>MHHHHHHMGDALGLIETKGLVACIEAADAMCDAANVELIGYENVGSGLVTAMVKGDVGAVKAAVDSGVESAQRIGEVVTSLVIARP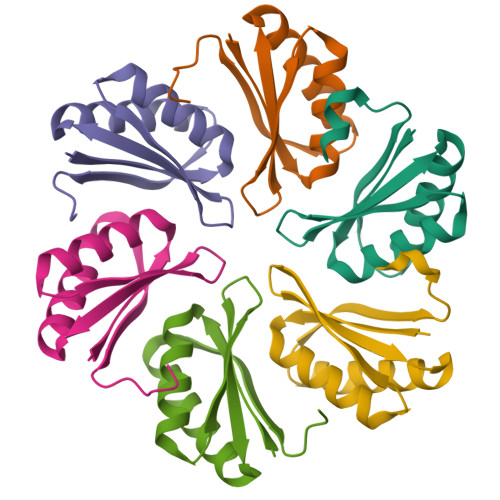HNDINKIVSHYKITD[6x]(1R,6S,7R,8S)-1-THIONIABICYCLO[4.3.0]NONAN-7,8-DIOL | C8 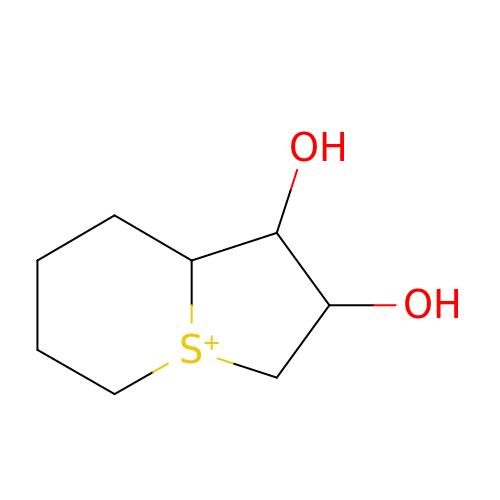H15 O2 S | CTIJTKTUZSCTEC-FBSDJGSXSA-N> MSDVAETLDPLRLPLQGERLIEASAGTGKTFTIAALYLRLLLGLGGSAAFPRPLTVEELLVVTFTEAATAELRGRIRSNIHELRIACLRETTDNPLYERLLEEIDDKAQAAQWLLLAERQMDEAAVFTIHGFCQRMLNLNAFESGMLFEQQLIEDESLLRYQACADFWRRHCYPLPREIAQVVFETWKGPQALLRDINRYLQGEAPVIKAPPPDDETLASRHAQIVARIDTVKQQWRDAVGELDALIESSGIDRRKFNRSNQAKWIDKISAWAEEETNSYQLPESLEKFSQRFLEDRTKAGGETPRHPLFEAIDQLLAEPLSIRDLVITRALAEIRETVAREKRRRGELGFDDMLSRLDSALRSESGEVLAAAIRTRFPVAMIDEFQDTDPQQYRIFRRIWHHQP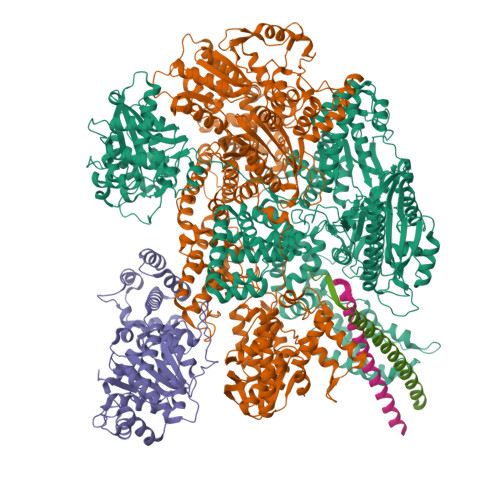ETALLLIGDPKQAIYAFRGADIFTYMKARSEVHAHYTLDTNWRSAPGMVNSVNKLFSQTDDAFMFREIPFIPVKSAGKNQALRFVFKGETQPAMKMWLMEGESCGVGDYQSTMAQVCAAQIRDWLQAGQRGEALLMNGDDARPVRASDISVLVRSRQEAAQVRDALTLLEIPSVYLSNRDSVFETLEAQEMLWLLQAVMTPERENTLRSALATSMMGLNALDIETLNNDEHAWDVVVEEFDGYRQIWRKRGVMPMLRALMSARNIAENLLATAGGERRLTDILHISELLQEAGTQLESEHALVRWLSQHILEPDSNASSQQMRLESDKHLVQIVTIHKSKGLEYPLVWLPFITNFRVQEQAFYHDRHSFEAVLDLNAAPESVDLAEAERLAEDLRLLYVALTRSVWHCSLGVAPLVRRRGDKKGDTDVHQSALGRLLQKGEPQDAAGLRTCIEALCDDDIAWQTAQTGDNQPWQVNDVSTAELNAKTLQRLPGDNWRVTSYSGLQQRGHGIAQDLMPRLDVDAAGVASVVEEPTLTPHQFPRGASPGTFLHSLFEDLDFTQPVDPNWVREKLELGGFESQWEPVLTEWITAVLQAPLNETGVSLSQLSARNKQVEMEFYLPISEPLIASQLDTLIRQFDPLSAGCPPLEFMQVRGMLKGFIDLVFRHEGRYYLLDYKSNWLGEDSSAYTQQAMAAAMQAHRYDLQYQLYTLALHRYLRHRIADYDYEHHFGGVIYLFLRGVDKEHPQQGIYTTRPNAGLIALMDEMFAGMTLEEA;> MLRVYHSNRLDVLEALMEFIVERERLDDPFEPEMILVQSTGMAQWLQMTLSQKFGIAANIDFPLPASFIWDMFVRVLPEIPKESAFNKQSMSWKLMTLLPQLLEREDFTLLRHYLTDDSDKRKLFQLSSKAADLFDQYLVYRPDWLAQWETGHLVEGLGEAQAWQAPLWKALVEYTHQLGQPRWHRANLYQRFIETLESATTCPPGLPSRVFICGISALPPVYLQALQALGKHIEIHLLFTNPCRYYWGDIKDPAYLAKLLTRQRRHSFEDRELPLFRDSENAGQLFNSDGEQDVGNPLLASWGKLGRDYIYLLSDLESSQELDAFVDVTPDNLLHNIQSDILELENRAVAGVNIEEFSRSDNKRPLDPLDSSITFHVCHSPQREVEVLHDRLLAMLEEDPTLTPRDIIVMVADIDSYSPFIQAVFGSAPADRYLPYAISDRRARQSHPVLEAFISLLSLPDSRFVSEDVLALLDVPVLAARFDITEEGLRYLRQWVNESGIRWGIDDDNVRELELPATGQHTWRFGLTRMLLGYAMESAQGEWQSVLPYDESSGLIAELVGHLASLLMQLNIWRRGLAQERPLEEWLPVCRDMLNAFFLPDAETEAAMTLIEQQWQAIIAEGLGAQYGDAVPLSLLRDELAQRLDQERISQRFLAGPVNICTLMPMRSIPFKVVCLLGMNDGVYPRQLAPLGFDLMSQKPKRGDRSRRDDDRYLFLEALISAQQKLYISYIGRSIQDNSERFPSVLVQELIDYIGQSHYLPGDEALNCDESEARVKAHLTCLHTRMPFDPQNYQPGERQSYAREWLPAASQAGKAHSEFVQPLPFTLPETVPLETLQRFWAHPVRAFFQMRLQVNFRTEDSEIPDTEPFILEGLSRYQINQQLLNALVEQDDAERLFRRFRAAGDLPYGAFGEIFWETQCQEMQQLADRVIACRQPGQSMEIDLACNGVQITGWLPQVQPDGLLRWRPSLLSVAQGMQLWLEHLVYCASGGNGESRLFLRKDGEWRFPPLAAEQALHYLSQLIEGYREGMSAPLLVLPESGGAWLKTCYDAQNDAMLDDDSTLQKARTKFLQAYEGNMMVRGEGDDIWYQRLWRQLTPETMEAIVEQSQRFLLPLFRFNQS;> MKLQKQLLEAVEHKQLRPLDVQFALTVAGDEHPAVTLAAALLSHDAGEGHVCLPLSRLENNEASHPLLATCVSEIGELQNWEECLLASQAVSRGDEPTPMILCGDRLYLNRMWCNERTVARFFNEVNHAIEVDEALLAQTLDKLFPVSDEINWQKVAAAVALTRRISVISGGPGTGKTTTVAKLLAALIQMADGERCRIRLAAPTGKAAARLTESLGKALRQLPLTDEQKKRIPEDASTLHRLLGAQPGSQRLRHHAGNPLHLDVLVVDEASMIDLPMMSRLIDALPDHARVIFLGDRDQLASVEAGAVLGDICAYANAGFTAERARQLSRLTGTHVPAGTGTEAASLRDSLCLLQKSYRFGSDSGIGQLAAAINRGDKTAVKTVFQQDFTDIEKRLLQSGEDYIAMLEEALAGYGRYLDLLQARAEPDLIIQAFNEYQLLCALREGPFGVAGLNERIEQFMQQKRKIHRHPHSRWYEGRPVMIARNDSALGLFNGDIGIALDRGQGTRVWFAMPDGNIKSVQPSRLPEHETTWAMTVHKSQGSEFDHAALILPSQRTPVVTRELVYTAVTRARRRLSLYADERILSAAIATRTERRSGLAALFSSRE;>[2x]MSRDLVTIPRDVWNDIQGYIDSLERENDSLKNQLMEADEYVAELEEKLNGTS>SNQAKADAVKEAFQHAWNGYMKYAFPHDELTPVSNGHADSRNGWGASAVDALSTAVIMGKADVVNAILEHVADIDFSKTSDTVSLFETTIRYLAGMLSGYDLLQGPAKNLVDNQDLIDGLLDQSRNLADVLKFAFDTPSGVPYNNINITSHGNDGATTNGLAVTGTLVLEWTRLSDLTGDEEYAKLSQKAESYLLKPQPSSSEPFPGLVGSSININDGQFADSRVSWNGGDDSFYEYLIKMYVYDPKRFETYKDRWVLAAESTIKHLKSHPKSRPDLTFLSSYSNRNYDLSSQHLTCFDGGSFLLGGTVLDRQDFIDF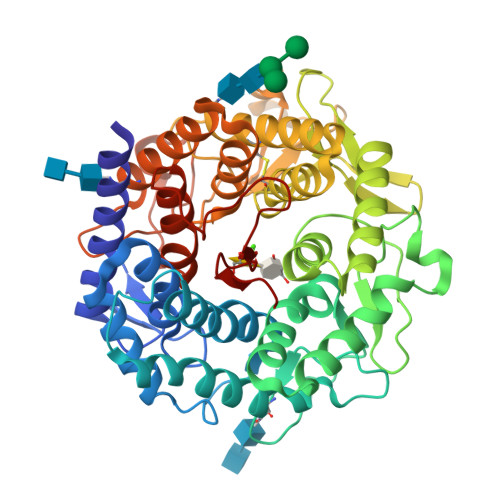GLELVDGCEATYNSTLTKIGPDSWGWDPKKVPSDQKEFYEKAGFYISSGSYVLRPEVIESFYYAHRVTGKEIYRDWVWNAFVAINSTCRTDSGFAAVSDVNKANGGSKYDNQESFLFAEVMKYSYLAHSEDAAWQVQKGGKNTFVYNTEAHPISVAR[2x]> AYFQGMVDVAFVCLGNICRSPMAEAIMRQRLKDRNIHDIKVHSRGTGSWNLGEPPHEGTQKILN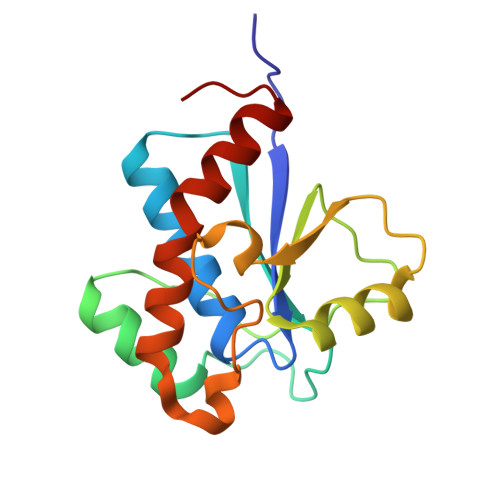KHNIPFDGMISELFEATDDFDYIVAMDQSNVDNIKSINPNLKGQLFKLLEFSNMEESDVPDPYYTNNFEGVYDMVLSSCDNLIDYIVKDANLKG> GPLGSEDDLYRQSLEIISRYLREQATGAKDTKPMGRSGATSRKALETLRRVGDGVQRNHETAFQGMLRKLDIKNEGDVKSFSRVMVHVFKDGVTNWGRIVTLISFGAFVAKHLKSVNQESFIEPLAETITDVLV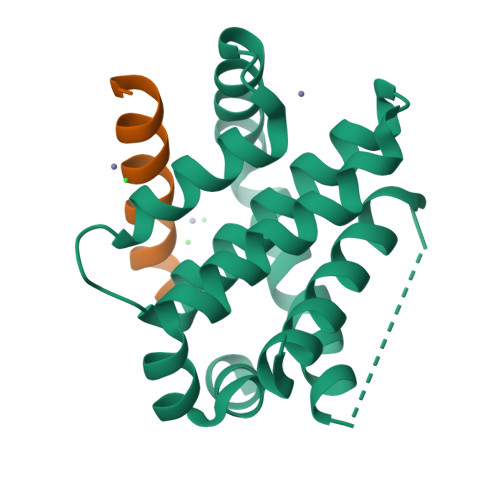RTKRDWLVKQRGWDGFVEFFHVQDLEGG;> RGEEEQWAREIGAQLRRMADDLN>GASMTLNQTTGPNLREQLIVSAHRWLSTMNDFTPDAMVSHRTEECVTRPAPRSLG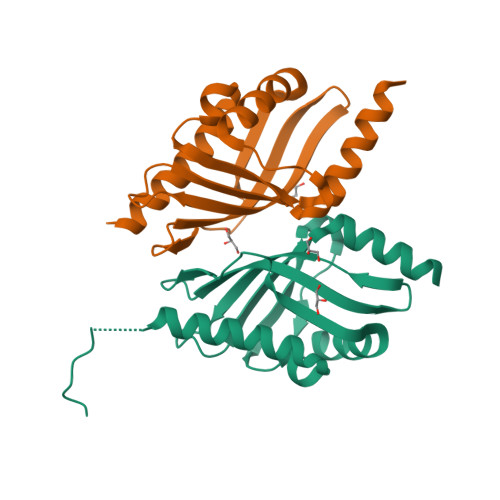FAPLNNGQLRTFFKTLTAQMKNFNLALMPGAVPIVDERLRKVVMHLASYAEAACGLYENEYMVVLTFNEEGTLLRDVIEFADSDYCVKFAERQAAAAESTSI[2x]> MSEQSICQARAAVMVYDDANKKWVPAGGSTGFSRVHIYHHTGNNTFRVVGR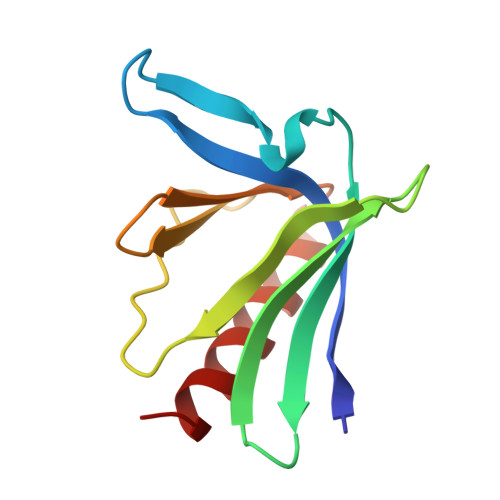KIQDHQVVINCAIPKGLKYNQATQTFHQWRDARQVYGLNFGSKEDANVFASAMMHALEVLN>MGHHHHHHHHHHHHSSGHIDDDDKHMLEMIQSHPLLAAPLAVGDTIGFFSSSAPATVTAKNRFFRGVEFLQRKGFKLVSGKLTGKTDFYRSGTIKERAQEFNELVYNPDITCIMSTIGGDNSNSLLPFLDYDAIIANPKIIIGYSDTTALLAGIYAKTGLITFYGPALIPSFGEHPPLVDITYESFIKILTRKQAGIYTYTLPEKWSDESINWNENKILRPKKLYKNNCAFYGSGKVEGRVIGGNLNTLTGIWGSEWMPEIRNGDILFIEDSRKSIATVERLFSMLKLNRVFDKVSAIILGKHELFDCAGSKRRPYEVLTEVLDGKQIPVLDG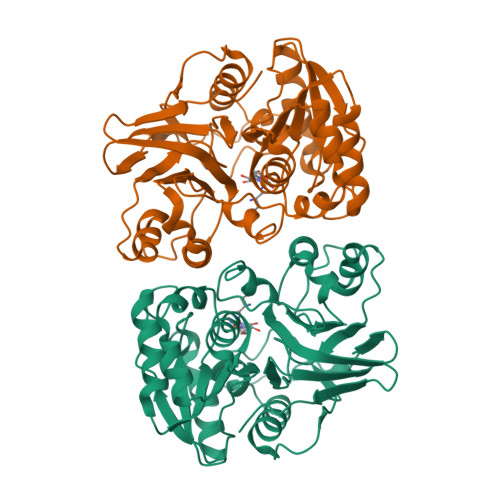FDCSHTHPMLTLPLGVKLAIDFDNKNISITEQYLSTEK[2x]> NDPGKMLKDAIDKQVAGALVAGTTTSTHSVATDSTPALQAAETGATSTARDESMIETRTIVPTHGIHETSVESFFGRSSLVGMP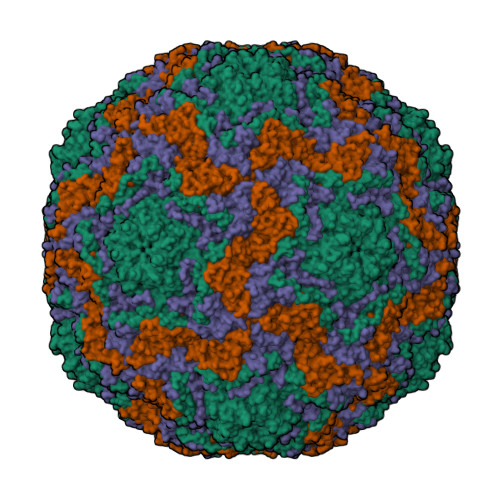LLATGTSITHWRIDFREFVQLRAKMSWFTYMRFDVEFTIIATSSTGQNVTTEQHTTYQVMYVPPGAPVPSNQDSFQWQSGCNPSVFADTDGPPAQFSVPFMSSANAYSTVYDGYARFMDTDPDRYGILPSNFLGFMYFRTLEDAAHQVRFRIYAKIKHTSCWIPRAPRQAPYKKRYNLVFSGDSDRICSNRASLTSY;> SPSAEACGYSDRVAQLTLGNSTITTQEAANICVAYGCWPAKLSDTDATSVDKPTEPGVSADRFYTLRSKPWQADSKGWYWKLPDALNNTGMFGQNAQFHYIYRGGWAVHVQCNATKFHQGTLLVLAIPEHQIATQEQPAFDRTMPGSEGGTFQEPFWLEDGTSLGNSLIYPHQWINLRTNNSATLILPYVNAIPMDSAIRHSNWTLAIIPVAPLKYAAETTPLVPITVTIAPMETEYNGLRRAIASNQ;> GLPTKPGPGSYQFMTTDEDCSPCILPDFQPTPEIFIPGKVNNLLEIAQVESILEANNREGVEGVERYVIPVSVQDALDAQIYALRLELGGSGPLSSSLLGTLAKHYTQWSGSVEITCMFTGTFMTTGKVLLAYTPPGGDMPRNREEAMLGTHVIWDFGLQSSITLVIPWISASHFRGVSNDDVLNYQYYAAGHVTIWYQTNMVIPPGFPNTAGIIMMIAAQPNFSFRIQKDREDMTQTAILQ;> GAQGGSTINYNNINYYSHAASAAQNKQDFTQDPSKFTQPIADVIKETAVPLK2-AMINO-7-[2-(2-HYDROXY-1-HYDROXYMETHYL-ETHYLAMINO)-ETHYL]-1,7-DIHYDRO-PURIN-6-ONE 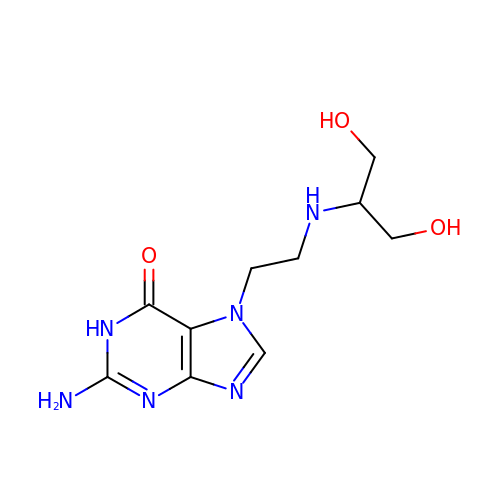| C10 H16 N6 O3 | XYCDSKWPYZSIDU-UHFFFAOYSA-N> GPLGSMKTILVKNLPSDTTQEEVLDYFSTIGPIKSVFISEKQANTPHKAFVTYKNEEESKKA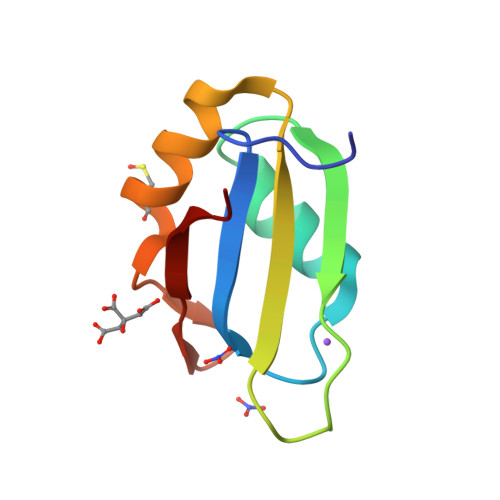QKCLNKTIFKNHTIWVGPGK>GPGMAVKHLIVLKFKDEITEAQKEEFFKTYVNLVNIIPAMKDVYWGKDVTQKNKEEGYTHIVEVTFESVETIQD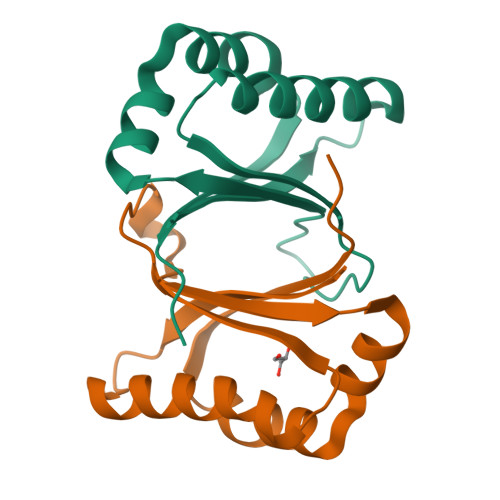FIIHPAHVGFGDVYRSFWEKLLIFDYTPRK[2x]> MSGQFTGTGTGGDVFKVDLNEQFDRADMVWIGTASVLVWIMIPGVGLLYSGISRKKHALSLMWAALMAACVAAFQWFWWGYSLVFAHNGSVFLGTLQNFCLKDVLGAPSIVKTVPDILFCLYQGMFAAVTAILMAGAGCERARLGPMMVFLFIWLTVVYCPIAYWTWGGNGWLVSLGALDFAGGGPVHENSGFAALAYSLWLGKRHDPVAKGKVPKYKPHSVSSIVMGTIFLWFGWYGFNGGSTGNSSMRSWYACVNTNLAAATGGLTWMLVDWFRTGGKWSTVGLCMGAIAGLVGITPAAGYVPVYTSVIFGIVPAIICNFAVDLKDLLQIDDGMDVWALHGVGGFVGNFMTGLFAADYVAMIDGTEIDGGWMNHHWKQLGYQLAGSCAVAAWSFTVTSIILLAMDRIPFLRIRLHEDEEMLGTDLAQIGEYAYYADDDPETNPYVLEPIRDTTISQPLPHIDGVADGSSNNDSGEAKNHHHHHH

structures of the Mep2 transceptors from S. cerevisiae and C. albicans. function as ammonium receptors/sensors in fungal development. a central channel for the transport of ammonium. non-phosphorylated, with channels that are closed on the cytoplasmic side.

structure of the ‘single D' S453D mutant. The channels of phosphorylation-mimicking mutants of C.> GSHMKTLIIYSSETGNTKMVCEKAFEYINGEKVIIPIKEEDSINLDEFDNIVVGTWIDKANANAEARKFINTLSNKKIFFIGTLAASLESEHAKKCFNNLTKLCSKKNNFVDGVLTRGKVSKDLQEKFTKFPLNIIHKFVPNMKEIILEADCHPNESDFLLIKGFIDKNFNY

We discovered that HmuF and a paralog, FldH, bind tightly to both FMN and heme. In contrast to flavodoxins, FldH and HmuF do not stabilize the FMN semiquinone but instead cycle between the FMN oxidized and hydroquinone states. We show that heme-loaded HmuF and heme-loaded FldH traffic heme to HmuW for degradation of the protoporphyrin ring. Both FldH and HmuF then catalyze multiple reductions of anaerobilin through hydride transfer from the FMN hydroquinone.

However, brown crystals of heme-bound FldH were obtained. The crystal structure was solved to a resolution of 1.6 Å. All of the 169 residues of FldH are present in the structure along with the heme and FMN cofactors. A notable feature of the structure is the helical cap domain (Lys116-His150) that bisects β5 and ⍺8 of the flavodoxin motif. This helical cap, comprising ⍺5, ⍺6, and ⍺7, provides a cleft for heme to be positioned planar to the si-face of the FMN isoalloxazine ring. The heme iron is coordinated on the proximal side by Nε of His134 in ⍺6 (Fe-Nε distance of 2.2 Å) and on the distal side by a water molecule, a coordination environment that is consistent with the electronic absorption spectrum of the heme-bound protein. The side chains of Leu121, Phe125, Leu130, Ile133, Val137, and Met140 form van der Waals interactions with the proximal side of the heme, creating a hydrophobic interface. An ion pair between the propionate group of the D pyrrole ring and the side chain of Lys92 (from ⍺3) further secures the heme to the protein. The orientation of the heme results in the B pyrrole ring forming pi-pi interactions with the pyrimidine ring of FMN. This places FMN N5, the site of hydride transfer, 3 Å from C5 of the tetrapyrrole ring (i.e., at the ⍺-meso bridge).>MALGTSGVKIHPNGNSNQLGVQLENVKLTSLFKKLDKRCSLASWIKENIKKKECCFYVEDGREGICKCGYPKVQHCDEAIKPEDYMGEQWDKHRHVRETPTDAFGDISFGGLGQKTGKYVRVSSDTSCENLYQLMTEQWKLRSPNLLISVTGGAKNFYIKTHLKDKFRRGLIKVAQTTGAWILTGGTHAGVMKHVGMAVRDYTLSSGSMEGQIVVIGVAPWGVIHNRSTLIHPEGRFPAYYSLDEQGQGRLSCLDINHTHFLLVDDGTQGHYGVEIELRARLEKLISKLSLGNRESGVTIPVVCVVLDGGPGTLNTIYNSMLNHTPCVVLEGSGRLADVIAHVASVPVSKVTMALINRLLKRFFMQEYKNFTELQIIEWTKKIQDILRMPHLLTVFRIDEDKNYDVDVAILQALLKASRSDEHAGRHCWERQLELAVAWNRVDIAESEIFTEESQWTSSDLHPAMFSALVGDK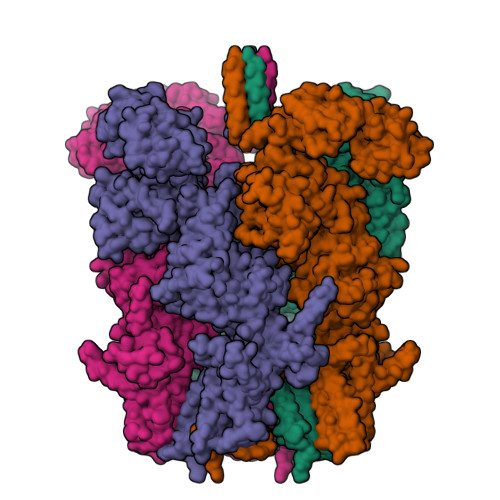PEFVRLLLENGVCVREFLEREETLCELYSHLPSCFFLRKLAKRVQGGKMRRGQEPLPGSRKVCLSHVSEEVRHLLGSFTQPLYIASRYKPTKDDVRLKVPSKGALDLPCSGEEWSADTVWDPGRDLFLWAVVQNNRELAEIGWEQCRDCIAAALAASKILRKLAQESGEDDSEEATEMLELANHYEKQAIGVFSECHSWDAQRAQKLLIRISPSWGRSTCLWLALEAHDKSFIAHSGVQALLTQIWCGELSVDNPHWKVLLCMIFFPLIYTGFLTFRRDEDIQRQAERTEQQKLAMESVFAGQSDGKIKRHLRGFSQKSELKPLNCSSRLMSFLKSPQVKFYWNIASYFGFLWLFAVVLMIDFQTSPSWRELLLYVWLTSLVCEEIRQLYHDFDGSGFRRKAKMYIKDLWNILDVLSIVLFIAGLICRLQASDTVFYIGKVILCIDFIIFCLRLMAIFSISRTLGPKIIIVRRMMLDLFFFMFLLSIWVVAYGVAKQGILIENEERLNWIIRGAVYEPYITIFGNFPTNIDNTLFDISSCSVNASDPLKPKCPMLNADNTPVFPEWLTIMMLCVYLLFANILLLNLLIAIFNYTFQEVQDNTDTIWKFQRYELIKEYHSRPALPPPFILLSHLILFIRGVFLRDLPQRHKNFRQELEQTEEEELLSWEAYMKDNYLASTRQDESQSVEHRIHDTAEKVGAMSELLEREQEMVXXXXXXXXXXXXXXXXXXXXXXDEEAPHMFARQLQYPDSTVRRFPVPEEKVSWEVNFSPYQPPVYNQQDSSESDTSALDKHRNPGGRTGIRGKGALNTLGPNHILHPIFTRWRDAEHKVLEFLAVWEDAEKRWALLGGPAQPDEPLAQVLERILGKKLNEKTKTLLKAGEEVYKGYVDDSRNTDNAWVETSIITLHCDKNTPLMADLNHMVESSLSSHQPLQWREVSSDACRCSYQREALRQIAHHHNTYFSNSLEVLFQGPDYKDDDDKAHHHHHHHHHH[4x]>MTADGPRELLQLRAAVRHRPQDFVAWLMLADAELGMGDTTAGEMAVQRGLALHPGHPEAVARLGRVRWTQQRHAEAAVLLQQASDAAPEHPGIALWLGHALEDAGQAEAAAAAYTRAHQLLPEEPYITAQLLNWRRRLCDWRALDVLSAQVRAAVAQGVGAVEPFAFLSEDASAAEQLACARTRAQAIAASVRPLAPTRVRSKGPLRVGFVSNGFGAHPTGLLTVALFEALQRRQPDLQMHLFATSGDDGSTLRTRLAQASTLHDVTALGHLATAKHIRHHGIDLLFDLRGWGGGGRPEVFALRPAPVQVNWLAYPGTSGAPWMDYVLGDAFALPPALEPFYSEHVLRLQGAFQPSDTSRVVAEPPSRTQCGLPEQGVVLCCFNNSYKLNPQSMARMLAVLREVPDSVLWLLSGPGEADARLRAFAHAQGVDAQRLVFMPKLPHPQYLARYRHADLFLDTHPYNAHTTASDALWTGCPVLTTPGETFAARVAGSLNHHLGLDEMNVADDAAFVA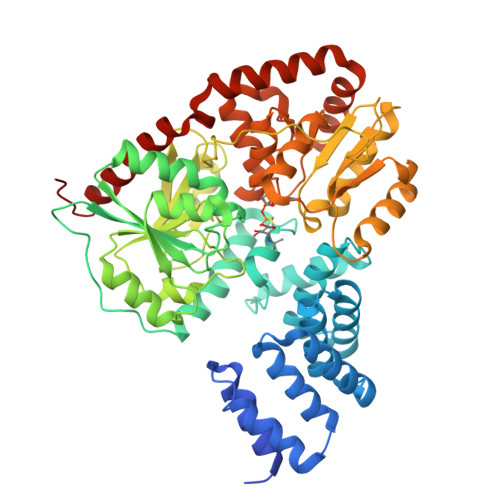KAVALASDPAALTALHARVDVLRRASGVFHMDGFADDFGALLQALARRHGWLGI[2x]>[4x]MAVSDSQNSQTCLDPDASRSVLGIILGGGAGTRLYPLTKKRAKPAVPLGANYRLIDIPVSNCLNSNISKIYVLTQFNSASLNRHLSRAYASNMGGYKNE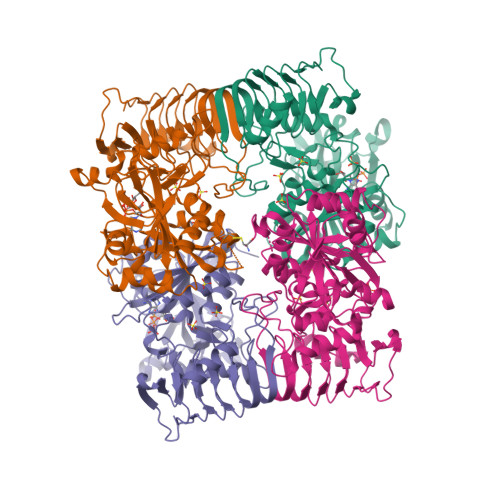GFVEVLAAQQSPENPDWFQGTADAVRQYLWLFEEHTVLEYLILAGDHLYRMDYEKFIQAHRETDADITVAALPMDEKRATAFGLMKIDEEGRIIEFAEKPQGEQLQAMKVDTTILGLDDKRAKEMPFIASMGIYVISKDVMLNLLRDKFPGANDFGSEVIPGATSLGMRVQAYLYDGYWEDIGTIEAFYNANLGITKKPVPDFSFYDRSAPIYTQPRYLPPSKMLDADVTDSVIGEGCVIKNCKIHHSVVGLRSCISEGAIIEDSLLMGADYYETDADRKLLAAKGSVPIGIGKNCHIKRAIIDKNARIGDNVKIINKDNVQEAARETDGYFIKSGIVTVIKDALIPSGIII> GGGRMATTTAGLTDLKFRVVREDFADAVAWVARSLPTRPTIPVLAGVLLTGTDEGLTISGFDYEVSAEVKVSAEIASAGSVLVS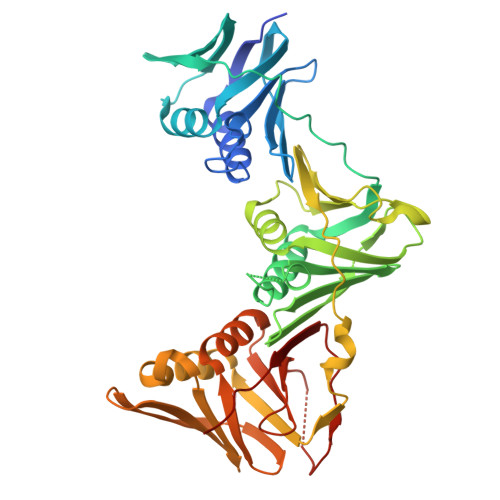GRLLSDITKALPAKPVEVSVEGTRVSLTCGSARFSLPTLAVEDYPALPALPEETGVIASDLFAEAIGQVAVAAGRDDTLPMLTGIRVEISGESVVLAATDRFRLAVRELTWVTTAGDVEAAVLVPAKTLAEAAKAGTDGNQVHLALGSGASVGKDGLLGIRSEGKRSTTRLLDAEFPKFRQLLPAEHTAVATIGVAELTEAIKRVALVADRGAQIRMEFSDDTLKLSAGADDVGRAEEDLPVDFAGEPLTIAFNPTYLTDGLGSLHSERVTFGFTTPSRPAVLRPAGEDDGANGGSGPFPAAKTDYVYLLMPVRLPG>ILPDSVDWREKGCVTEVKYQGSCGASWAFSAVGALEAQLKLKTGKLVSLSAQNLVDCSTEKYGNKGCNGGFMTTAFQYIIDNKGIDSDASYPYKAMDQKCQYDSKYRAATCSKYTELPYGREDVLKEAVANKGPVSVGVDARHPSFFLYRSGVYYEPSCTQNVNHGVLVVGYGD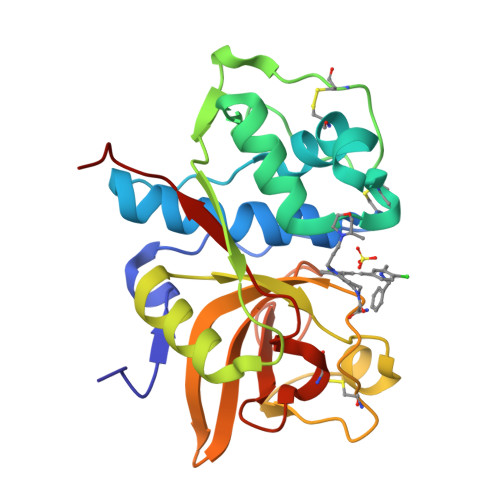LNGKEYWLVKNSWGHNFGEEGYIRMARNKGNHCGIASFPSYPEILQGGG[4x]> MSQVHIFWGAPIAPLKGSGSGSGSGSGSGS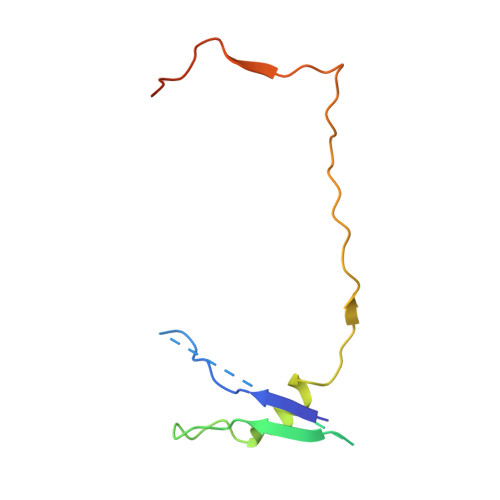GSTTEVILHYRPCESDPTQLPKIAEKAIQDFPTRPLSRFIPWFPYDGSKLPLRPKRSPPASREEIMATL> SGFTVKPVATVHRRIPDLPDCDIDKWLNNFNVPSPLNWERKIFSNCNFNLSTLLRLVHTDSFSCNNFDESKIYGSCFKSIVLDKFAIPNSRRSDLQLGSSGFLQSSNYKIDTTSSSCQLYYSLPAINVTINNYNPSSWNRRYGFNNFNLSSHSVVYSRYCFSVNNTFCPCAKPSFASSCKSHKPPSASCPIGTNYRSCESTTVLDHTDWCRCSCLPDPITAYDPRSCSQKKSLVGVGEHCAGFGVDEEKCGVLDGSYNVSCLCSTDAFLGWSYDTCVSNNRCNIFSNFILNGINSGTTCSNDLLQPNTEVFTDVCVDYDLYGITGQGIFKEVSAVYYNSWQNLLYDSNGNIIGFKDFVTNKTYNIFPCYAG;> MGSKCSNSGIECDS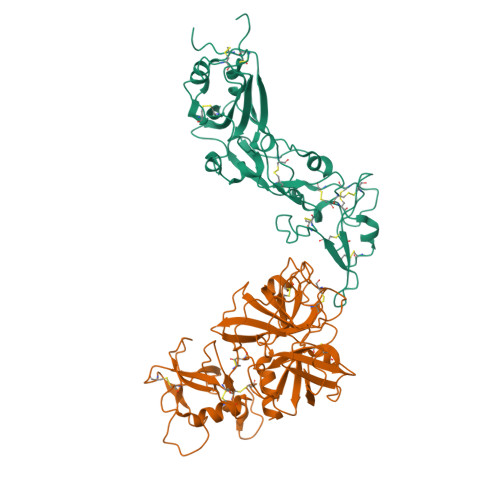SGTCINPSNWCDGVSHCPGGEDENRCVRLYGPNFILQVYSSQRKSWHPVCQDDWNENYGRAACRDMGYKNNFYSSQGIVDDSGSTSFMKLNTSAGNVDIYKKLYHSDACSSKAVVSLRCIACGVNLNSSRQSRIVGGESALPGAWPWQVSLHVQNVHVCGGSIITPEWIVTAAHCVEKPLNNPWHWTAFAGILRQSFMFYGAGYQVEKVISHPNYDSKTKNNDIALMKLQKPLTFNDLVKPVCLPNPGMMLQPEQLCWISGWGATEEKGKTSEVLNAAKVLLIETQRCNSRYVYDNLITPAMICAGFLQGNVDSCQGDAGGPLVTSKNNIWWLIGDTSWGSGCAKAYRPGVYGNVMVFTDWIYRQMRADG> DRVRNLQSEVEGVKNIMTQNVERILARGENLEHLRNKTEDLEATSEHFKTTSQKVARKFWWKNV;> ESWETLEADLIELSQLVTDFSLLVNSQQEKIDSIADHVNSAAVNVEEGTKNLGKAAKY;> ADRQQYLRQEVLRRAEATAASTSRSLALMYESEKVGVASSEELARQRGVLERTEKMVDKMDQDLKISQKHINSIKSVF;> HLRAYHQKIDSNLDELSMGLGRLKDIALGMQTEIEEQDDILDRLTTKV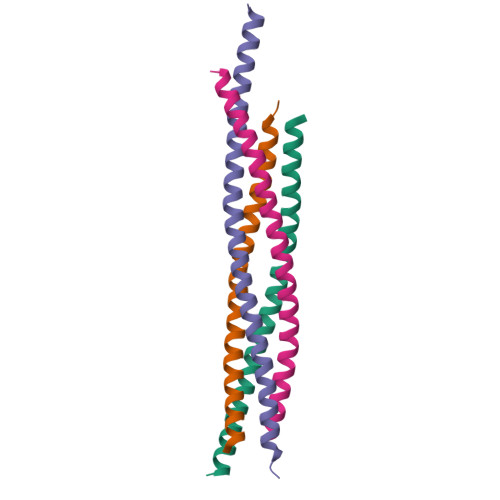DKLDVNIKSTERKVRQL> XFTGVQGRVIGYDILRSPEVDKAKPLFTETQWDGSELPIYDAKPLQDAL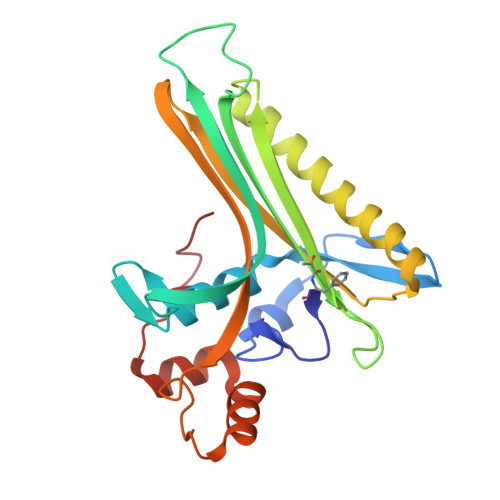VEYFGTEQDRRHYPAPGSFIVCANKGVTAERPKNDADMKPGQGYGVWSAIAISFAKDPTKDSSMFVEDAGVWETPNEDELLEYLEGRRKAMAKSIAECGQDAHASFESSWIGFAYTMMEPGQIGNAITVAPYVSLPIDSIPGGSILTPDKDMEIMENLTMPEWLEKMGYKSLSANNALKY>[6x]ALKRKIEAAKMPKDAREKTEAELQKLKMMSPMSAEATVVRGYIDWMLQVPWNSRSKVKKDLVKAQEVLDTDHYGLERVKDRILEYLAVQSRVSKIKGPILCLVGPPGVGKTSLGQSIAKATGRQYVRMALGGVRDEAEIRGHRRTYIGSMPGKLIQKMAKVGVKNPLFLLDQIDKMASDMRGDPASALLEVLDPEQNVAFNDHYLEVDYDLSDVMFVATSNSMNIPAPLLDRMEVIRLSGYTEDEKLNIAKQHLLPKQFERNAIKKGELTIDDSAIMSIIRYYTREAGVRSLEREISKLCRKAVKNLLMDKTVKHIEINGDNLKDFLGVQKVDYGRADTENRVGQVTGLAWTEVGGDLLTIETACVPGKGKLTYTGSLGEVMQESIQAALTVVRARADKLGINPDFYEKRDIHVHVPEGATPKDGPSAGIAMCTALVSCLTGNPVRADVAMTGEITLRGLV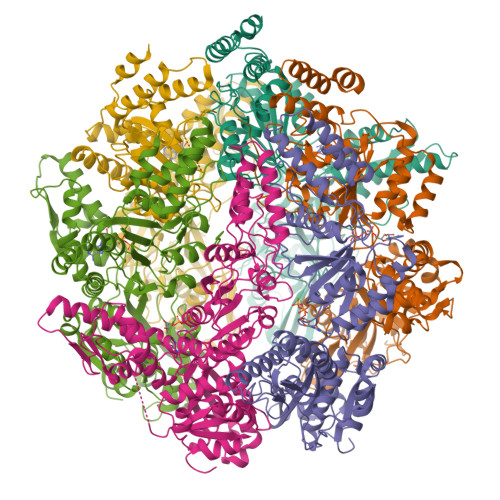LPIGGLKEKLLAAHRGGIKVVLIPDDNKRDLEEIPDNVIADLEIHPVKRIDDVLAIALEHPAF;> AAAAAAA>GPGVDEALREAQTKSAMNFIKDNSRALIQRMGMTVIKQITDDLFVWNVLNREEVNIICCEKVEQDAA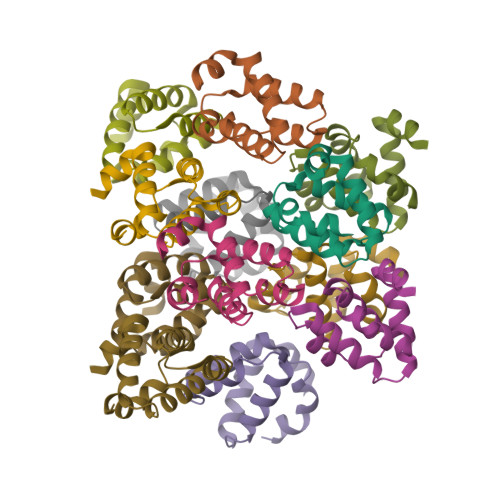RGIIHMILKKGSESCNLFLKSLKEWNYPLFQDLN[12x]>[2x]MMIIVGVDAGGTKTKAVAYDCEGNFIGEGSSGPGNYHNVGLTRAIENIKEAVKIAAKGEADVVGMGVAGLDSKFDWENFTPLASLIAPKVIIQHDGVIALFAETLGEPGVVVIAGTGSVVEGYNGKEFLRVGGRGWLLSDDGSAYWVGRKALRKVLKMMDGLENKTILYNKVLKTINVKDLDELVMWSYTSSCQIDLVASIAKAVDEAANEGDTVAMDIL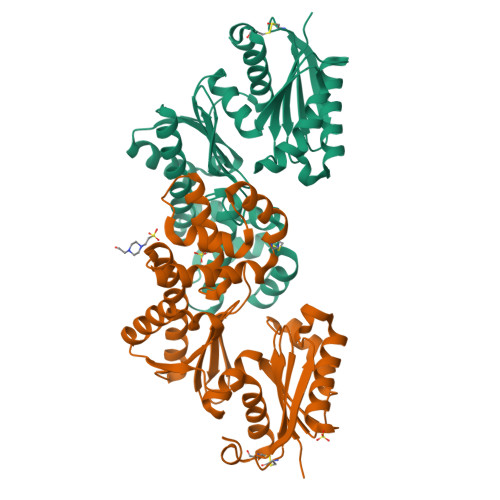KQGAELLASQAVYLARKIGTNKVYLKGGMFRSNIYHKFFTLYLEKEGIISDLGKRSPEIGAVILAYKEVGCDIKKLISD>GAMGMNTPPELDTVLQAPYAYN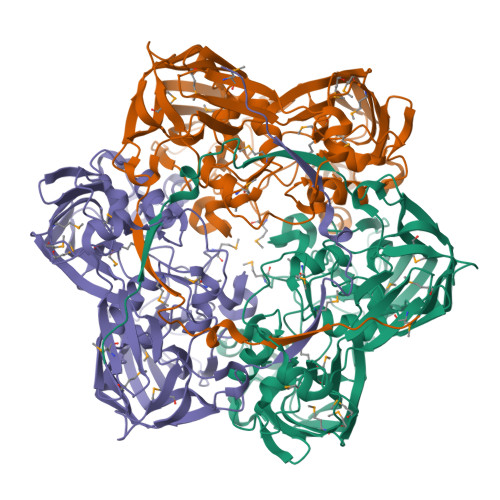WPTSKNVKIASRIGIPYSTFQTIQPVSDAPNNGIGQITFNQPLGNLTGGAPRLRVSFTAEIKNILADSSLKDQIGLKSFPVNRSIPVAVINMNGKTFTSYPAQLIKLHQYNADPLELALLSPCSDVDEYNKIKAVSMNNPYRQGTESTDSRMSRGLGCNYAYYIHPRAAGSTSVKIDFVVDEALVANPTQYKNIKDPVPFRNLNTFKVILDGQFKPENMIGIADDVKLVAGKADFEVDITGFKINMLVQNWVAPLEIGDIPKTIIYNTPLISLEGNISSMCLNTKDPYGIPGERNKHILTTHSMAMNNVPSMFAVMVSQETPTKKFAPDQLAGIIGLEIKVDSDVGIFRELEQQQLYELSSSNGYNKRFSCFSGALANGLTVADPAVAAGNKFKEAIFGAGSVIFFRPSDLGLKDYNVMANANKSINMQVQATFVTPEAAGTGAHYKLEVFSIRDNLTYSFEDGTFMDDLTLYTPDQLLRSPLKLTDDNNKLMRVMGG[3x]2-[2-(3-chloranyl-4-methoxy-phenyl)ethyl]-~{N}-cyclohexyl-7-(3,5-dimethyl-1,2-oxazol-4-yl)imidazo[1,2-a]pyridin-3-amine 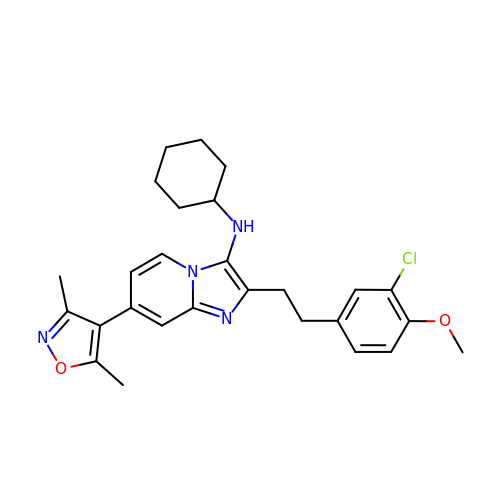| C27 H31 Cl N4 O2 | NZXSWCLCRDCHGN-UHFFFAOYSA-N In non-spherical bacteria, the actin homologue MreB is essential for shape maintenance as depletion of MreB through genetic knockouts or MreB-targeted drug treatment results in misshapen cells that eventually lyse. The MreB fibres are attached to the cell membrane via a hydrophobic loop in Thermotoga maritima as well as Gram+ bacteria and via an additional N-terminal amphipathic helix in Gram− bacteria. Here, we demonstrate that MreB from Caulobacter crescentus forms pairs of antiparallel protofilaments as revealed by crystal structures, an architecture unprecedented among actin-like proteins. The crystal structure of Caulobacter MreB (ΔCcMreBdh) reveals the typical actin fold, containing two domains on either side of a nucleotide binding cleft (Kabsch and Holmes, 1995).

A single mutation in the intra-protofilament interface (S283D, ΔCcMreBdmh) renders the protein monomeric, as shown both by crystallography and by EM. This mutant turned out to be most useful in studying the polymerisation cycle. Monomeric CcMreB shows little structural movement between the ADP- and the ATP analogue AMPPNP-bound states with domains I and II overlapping with an RMSD of 1.58 and 0.57 Å, respectively. (D) Superposition of ADP-bound ΔCcMreBdmh (m_2, shown in orange) and AMPPNP-bound ΔCcMreBdmh (m_3, shown in blue). A small movement of domain IB initiates the propeller twist observed upon polymerisation.

> MISNDIAIDLGTANTLIYQKGKGIVLNEPSVVALRNVGGRKVVHAVGIEAKQMLGRTPGHMEAIRPMRDGVIADFEVAEEMIKYFIRKVHNRKGSGNPKVIVCVPSGATAVERRAINDSCLNAGARRVGLIDEPMAAAIGAGLPIHEPTGSMVVDIGGGTTEVAVLSLSGIVYSRSVRVGGDKMDEAIISYMRRHHNLLIGETTAERIKKEIGTARAPADGEGLSIDVKGRDLMQGVPREVRISEKQAADALAEPVGQIVEAVKVALEATPPELADDIADKGIMLTGGGALLRGLDAEIRDHTGLPVTVADDPLSCVALGCGKVLEHPKWMKGVLESTLAGSHHHHHH> YPGGS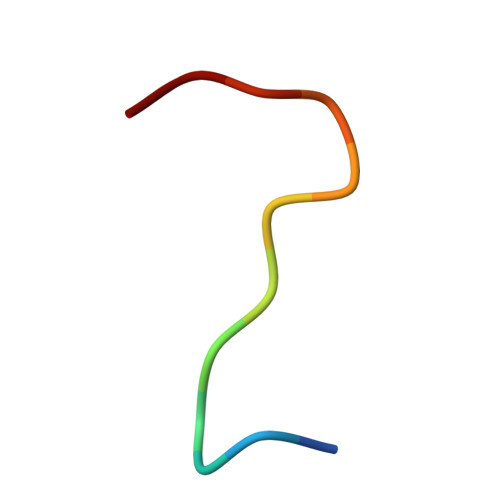FDPLGLA>MSSCKDSLSLMAMWGSIARFDPKHERSFEGPEKRLEVIMRVVDGTHVSGLLAHDDDVWQKVIDAICAHIVSREFNEYIRSYVLSE[2x];>[2x]XSLFVMKDRVILITCGTITLLNCVPLICEAVSTVCGEVEWVSFMHKNYSFPWEQKGPHLSMAEEFKTLRSHFPSGQPFIFGPIDSDHYFLYFHSDVVQPSCSDDAQLSMTMYGLDRNQTKHWYSDKMLPTGPETAVIREATGLSEVVDDSWILHDLQYEPCGYSINAIRGSEYQTIHITPEEHCSFASYETNTCALNYSKCICGVLRVFDPERFSVIVFIDPDSAVGKSYHSGGTIGVEPEYYPNYEAHHRTVNEYTPGHWVLKVNYVKRAVGTVGTSAASGAKE;>[2x]MSVTRINQQTECPSSVHDLVSCWGGCTQSKTSTDSGLEKRFELNFAQPVDIGTVTVKQLASVMERAGESLRQNSAELGIHTLKFDRSLLVFTAKQIVVRSSVSVMLHEAVHPMLELMRSHNIIVDWASFMRVNYGSPWDMTSETSDIMAHEYAELKSAFPTGHPYLAGPVDRDHCFYFVYDGIDRDPSSCRRENDVQINVYMYNVQADDEYDLDGNTKEQQLLVSHCAGEYETLRVSTYGSTHPFASFETNAVSAASDITKIVNGLLKKFYPERVLLVLLQDRDAQGTTACGVMDRLEGFTVVHRGANHFGGGYVFHQATYARSA

AdoMetDC is a pyruvoyl-dependent enzyme that catalyzes formation of decarboxylated AdoMet, a substrate required for biosynthesis of the polyamine spermidine from putrescine. The AdoMetDC pyruvoyl group plays a key role in the catalytic mechanism and derives from an autocatalytic processing reaction that cleaves the peptide backbone into β- and α-chains. Trypanosomatid AdoMetDC undergoes this cleavage, while the corresponding pseudoenzyme, which we call ‘prozyme’, lacks key residues and is not processed to the active form.

TbAdoMetDC/prozyme wild-type heterodimer was crystallized with putrescine both in the absence (apo-TbAdoMetDC/prozyme) and presence (CGP-TbAdoMetDC/prozyme) of CGP 40215 (CGP), a known AdoMetDC inhibitor. The CGP-TbAdoMetDC/prozyme structure additionally has CGP bound in the active site and a second putrescine (Put) found in a novel site near the N-terminal α-helix (h1). Comparison of CGP-TbAdoMetDC/prozyme heterodimer with the apo-TbAdoMetDC/prozyme structure shows that conformational changes upon ligand binding are limited to the movement of a couple of residues in the flexible connector arm (e.g. R26) adjacent to h1 and the active site. In the presence of ligand R26 repositions to form an interaction with the π electrons in the benzamidine ring of the inhibitor. CGP binds in the TbAdoMetDC active site with one amidine group buried 3.6 Å above the active site pyruvoyl group. CGP forms H-bonds with the backbone carbonyl of L83, the side chain hydroxyls of S249 and Y243, and with C100, suggesting C100 may be unprotonated leading to formation of an ion pair with the amidine of the inhibitor. The buried benzyl ring is sandwiched between Y243 and F28 forming π-π stacking interactions with the former and the guanidine group nitrogens (N01 and N03) form a bidentate H-bond with E266. The amidine of the second benzamidine group is solvent exposed. Furthermore, the active conformation is likely stabilized and perhaps regulated by pathway metabolites since putrescine is bound in the h1 helix pocket forming H-bonds with both h1 residues and residues forming the h1 binding pocket, such as H172. The fully activated T. brucei enzyme has a conformation and active site structure similar to the human enzyme however two residues within the 4 Å CGP 402015 inhibitor contacting surface differ between the human and T. brucei structures (TbR26/HsH5 and TbY243/HsF223).> GSHTAEEDMEDDTSWRSEATFQFTVERFSRLSESVLSPPCFVRNLPWKIMVMPRF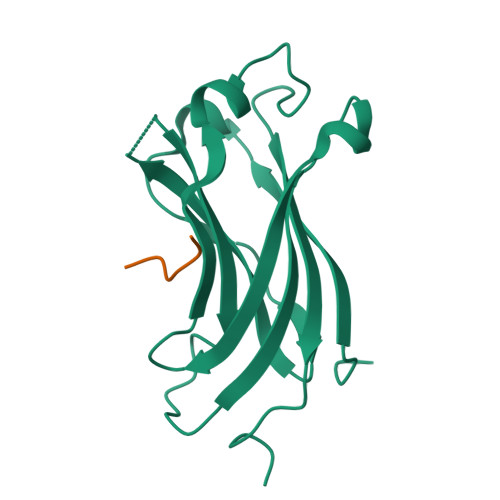YPDRPHQKSVGFFLQCNAESDSTSWSCHAQAVLKIINYRDDEKSFSRRISHLFFHKENDWGFSNFMAWSEVTDPEKGFIDDDKVTFEVFVQADAPHGVAW;> EPGGSR P. gingivalis displays two forms of fimbriae on its surface, FimA and Mfa1, both of which are crucial for attachment to other bacteria in the oral biofilm and to the host cells. In the work presented herein we have determined the crystal structures of the shaft protein Mfa1, in both mature and precursor forms, the anchor protein Mfa2 and a truncated precursor form of the tip protein, Mfa3. The resulting mature protein thereby has an empty position in the first β-sheet that a β-strand donated from another fimbrial protein presumably fills in order to polymerize the individual proteins into a polymeric fimbria.

The anchor protein Mfa2 does not contain any Rgp/Kgp processing sites and is in contrast to Mfa1 and Mfa3 considered to begin its mature sequence at the lipidated cysteine (Cys29) directly following the signal peptide. The full mature form, ranging from residues 29–324 was expressed, purified and crystallized. The final Mfa2 model consists of residues 40–320, and is built up from two β-sandwich domains (N- and C-domain) and measures 85 × 35 × 25 Å in size. Importantly, Mfa2 is stabilised by two disulphide bonds, a feature not present in Mfa1, Mfa3 or Mfa425. The first is formed between Cys54 and Cys285 and links the long β1β2-loop of the N-domain with a loop from the C-domain at the domain interface. The second disulphide is observed between Cys298 and Cys300, rigidifying the turn leading up to the penultimate and ultimate strands of the structure. In Mfa2 the equivalent residues are Val44, Val46 and Phe48. In the regulatory protein Mfa2, the C-terminus forms a final β-strand that following a β-hairpin runs antiparallel to the preceding strand. Whereas the Trps in Mfa1 and Mfa3 are firmly anchored in similar pockets, the equivalent Trp of Mfa2 (W315) is solvent exposed, due to the bend between the two last β-strands.

> CPRGVYVNFYSQTECAENPSYPAEVARLNVYAFDKDGILRSANVFEDVQLSAAKEWLIPLEKDGLYTIFAWGNIDDHYNIGEIKIGETTKQQVLMRLKQDGKWATNIDGTTLWYATSPVVELKNMEDGADQYIHTRANLREYTNRVTVSVDSLPHPENYEIKLASSNGSYRFDGTVAKADSTYYPGETKVVGDSTCRAFFTTLKLESGHENTLSVTHKPTGREIFRTDLVGAILSSQYAQNINLRCINDFDIRLVAHHCNCPDDTYVVVQIWINGWLIHSY>[4x]GPGSMAFDPNYPRDLIGYGRHPVQANWPGRARVAVQFVLNYEEGGENCVLHGDPASEQFLSEIVGAAAYPARHMSMESIYEYGSRAGVWRILREFDKRGLPLTVFGVGMAIERHPELARAFVELGHEIACHGWRWIHYQDMTPEREAEHMRLGMEAIERVTGVRPLGWYTGRDSPNT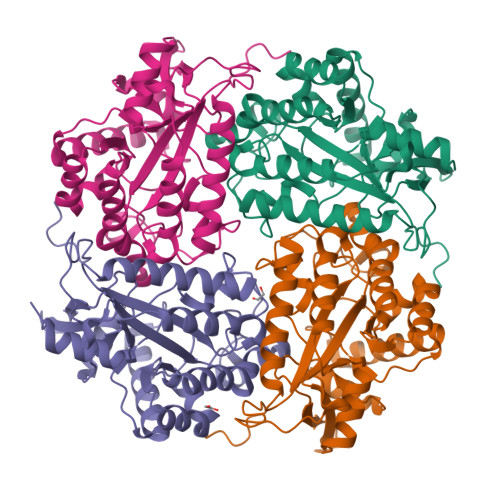HRLVAEYGGFLYDSDHYGDDLPFWMDVEVSGGASVPQLIVPYTLDANDMRFATPQGFNTADHFFHYLRDAFDVLYEEGDEAPKMMSIGMHCRLLGRPGRFRALQRFLDHIERHDRVWVARRVEIARHWREHHPYRPHARREGDA> ATTDAECLSKPAFDGTLSNVWKEGDSRYANFENCIYELSG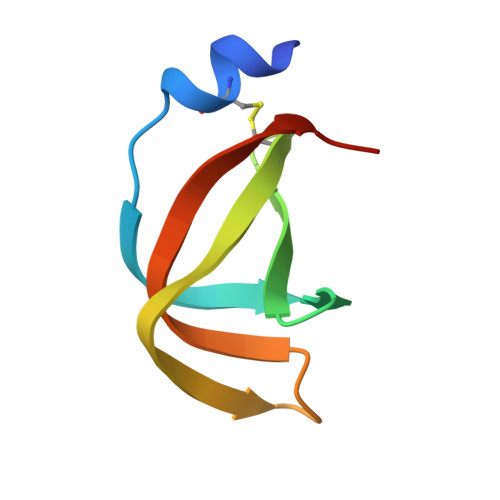IGIGYDNDTSWNGHWTPVRAADGSG> MSGGDTRAAIARPRMAAAHGPVAPSSPEQNGAVPSEATKRDQNLKRGNWGNQIEFVLTSVGYAVGLGNVWRFPYLCYRNGGGAFMFPYFIMLIFCGIPLFFMELSFGQFASQGCLGVWRISPMFKGVGYGMMVVSTYIGIYYNVVICIAFYYFFSSMTHVLPWAYCNNPWNTHDCAGVLDASNLTNGSRPAALPSNLSHLLNHSLQRTSPSEEYWRLYVLKLSDDIGNFGEVRLPLLGCLGVSWLVVFLCLIRGVKSSGKVVYFTATFPYVVLTILFVRGVTLEGAFDGIMYYLTPQWDKILEAKVWGDAASQIFYSLGCAWGGLITMASYNKFHNNCYRDSVIISITNCATSVYAGFVIFSILGFMANHLGVDVSRVADHGPGLAFVAYPEALTLLPISPLWSLLFFFMLILLGLGTQFCLLETLVTAIVDEVGNEWILQKKTYVTLGVAVAGFLLGIPLTSQAGIYWLLLMDNYAASFSLVVISCIMCVAIMYIYGHRNYFQDIQMMLGFPPPLFFQICWRFVSPAIIFFILVFTVIQYQPITYNHYQYPGWAVAIGFLMALSSVLCIPLYAMFRLCRTDGDTLLQRLKNATKPSRDWGPALLEHRTGRYAPTIAPSPEDGFEVQPL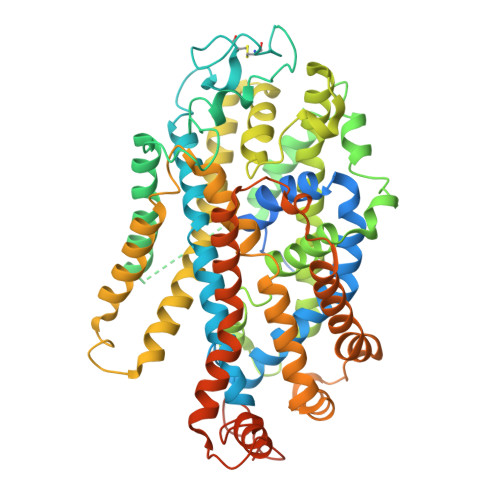HPDKAQIPIVGSNGSSRLQDSRI> AQEPVKGPVSTK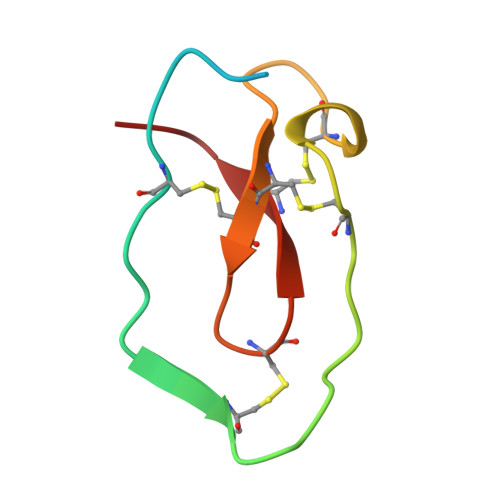PGSCPIILIRCAMLNPPNRCLKDTDCPGIKKCCEGSCGMACFVPQ>HHHHHHFNLPPGNYKKPVLLYCSNGGHFLRILPDGTVDGTRDRSDQHIQLQLSAESVGEVYIKSTETGQYLAMDTDGLLYGSQTPNEECLFLERLEENHYNTYISKKHAEKNWFVGLKKNGSVKRGPRTHYGQKAILFLPLPVSSD[2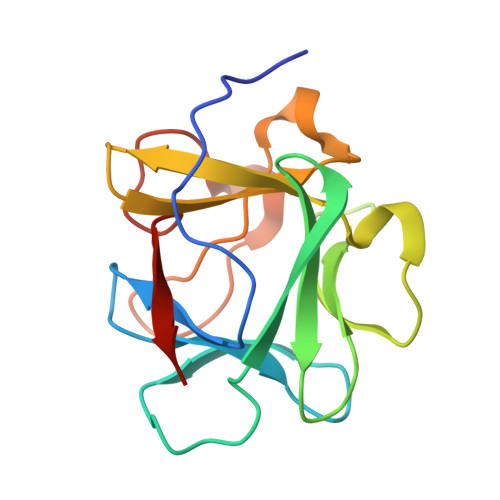x]1-[4-cyclopentyl-2-methyl-5-(2-piperazin-1-yl-1,3-thiazol-4-yl)-1~{H}-pyrrol-3-yl]ethanone 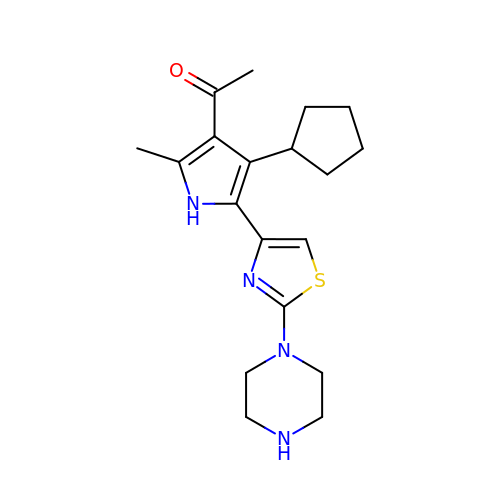| C19 H26 N4 O S | HIQSGTMYVPXYRT-UHFFFAOYSA-N> HKILHR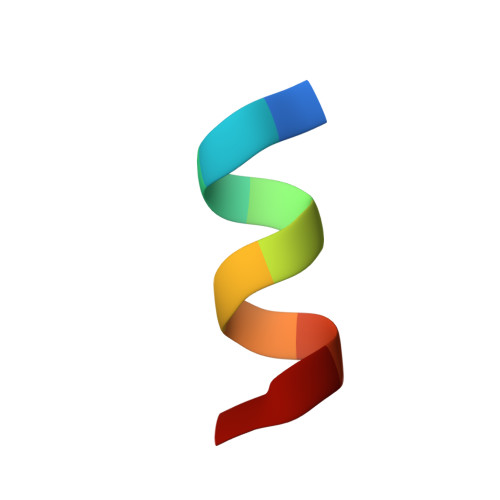LLQE> MFERFTDRARRVVVLAQEEARMLNHNYIGTEHILLGLIHEGEGVAAKSLESLGISLEGVRSQVEEIIGQGQQAPSGHIPFTPR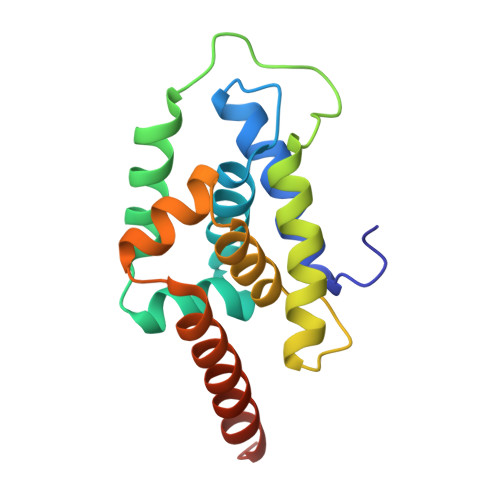AKKVLELSLREALQLGHNYIGTEHILLGLIREGEGVAAQVLVKLGAELTRVRQQVIQLLSGYKLAAALEHHHHHH>MRLPDPYTNPEYPGLGFESVNLVDNDPMIRDELPNGKVKEVKISAQYWGINISYPELFPDEYAFLDSRLLEYKRTGDYLDVLLPQYEAFRVRGDTKSVTIPAGQKGSQIILNTNGTLTGQPKAGDLFKLSTHPKVYKIT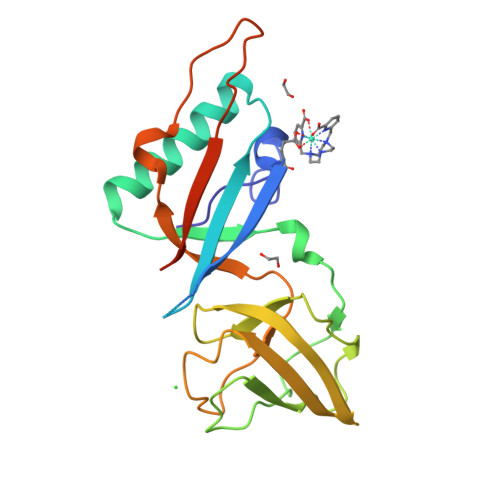NFSSSGNVWNISLYPDLFITTTGSEKPVFNGILFRTKLMNGDSFGSTLNNNGTYSGISLSLRESLENLYFQGHHHHHH[4x]>[2x]SEKYDGEWNEGRMQGWGKYFYADGGVYEGEWVDGRMHGRGTYVFPNGNKYEGEWVEDRKDGYGILLYTNGERYEGYWHLDKAHGKGTLTFLQGDRYVGEWHYGKKHGHGVLSYSNGDTYDGEWRDDDAWGYGVLQYANGCRYEGEWAEDRRHGKGLLVLPDGSSYEGSFAHGKKDGPGKIILKDGSMYIGTWKDGVIVGQGEFRLSENCDLSNPDY

High-resolution crystal structures and biophysical analyses of a truncated form of the TbMORN1 protein and its homologues from the parasites Toxoplasma gondii (TgMORN1) and Plasmodium falciparum (PfMORN1) enabled, for the first time, a structure-based definition of the MORN repeat. All three structures are antiparallel dimers joined via their C-termini, and, when possessed of the correct key residues, can adopt extended or V-shaped quaternary structures. The crystal structures confirmed that each 23-amino acid MORN repeat is composed of a β-hairpin followed by a 6-residue loop that connects to the next MORN repeat. The structural studies presented here make a case that one conserved function of MORN repeats is in homotypic interactions and possibly also in higher-order assembly.

The structures of TgMORN1(7–15) and both P21 and C2 crystal forms of TbMORN1(7–15) were subsequently determined to 2.90, 2.35 and 2.53 Å resolution, respectively, with the PfMORN1(7–15) structure used as a search model for the molecular replacement. The two subunits in the TbMORN1(7–15) C2 crystal form and the TgMORN1(7–15) dimer make a rather straight assembly, while in the P21 form they display a bend of about 30°, leading to a rod-shaped particle appearance. In contrast to the other two proteins, the P21 crystal structure of TbMORN1(7–15) displays a bend of approximately 30° among the sub-units. Superimposing the TbMORN1(7–15) P21 subunit with the structures of the TgMORN1(7–15) and PfMORN1(7–15) subunits over 202 Cα atoms yielded rmsd values of 1.0 and 1.1 Å, respectively, revealing high structural similarity between the three proteins. In the P21 and C2 TbMORN1(7–15) crystal forms, the dimer interfaces occupy surface areas of 747 Å2 and 966 Å2, respectively. Calculations of gain in solvation free energy (ΔiG) upon dimer formation for TbMORN1(7–15) C2 and P21 performed with the PDBePISA package yielded values of -20.1 kcal/mol and -11.3 kcal/mol, respectively, with corresponding p-values of interface specificity 0.01 and 0.08. ΔiG values lower than -10 to -15 kcal/mol and p-values lower than 0.5 are significant for stable protein dimers, indicating highly specific dimerisation interfaces. In the P21 crystal structure, the position of the loop differs from that in the C2 dimer and keeps the Cα atoms of Cys351 and Cys282 at a distance of 11.7 Å, preventing disulphide bond formation. Here, the side chain of Cys351 is engaged in a polar interaction with Asp303. (A) Conservation map of the TbMORN1(7–15) P21 crystal structure reveals a highly conserved stretch of residues along the groove. Analysis of the interaction and electrostatic maps of TbMORN1(7–15) and its mutagenised variants clearly showed that Arg293 and Lys316, residing in repeats 13 and 14 respectively, are crucial for maintaining TbMORN1 in a stable dimeric state through electrostatic interactions.>MRVIVFFDLPVITPENRHNYSVFRKYLIKSGFIMQQKSVYSKLVLNLTNRDSIVKSIEKNKPPEGLVEVLTVTEKQYAKMEIIIGESKTEYLN[2x];>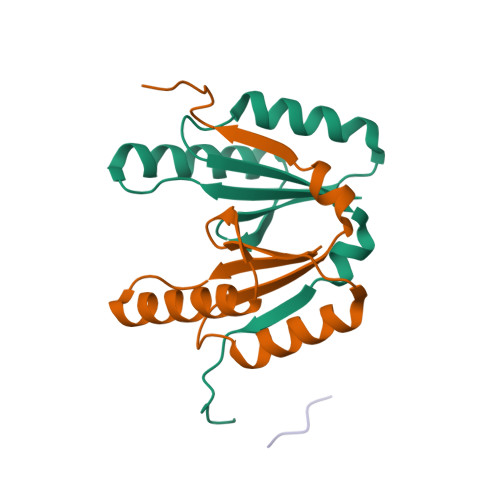 GGGGG3-(azepan-1-ylmethyl)-1~{H}-indole 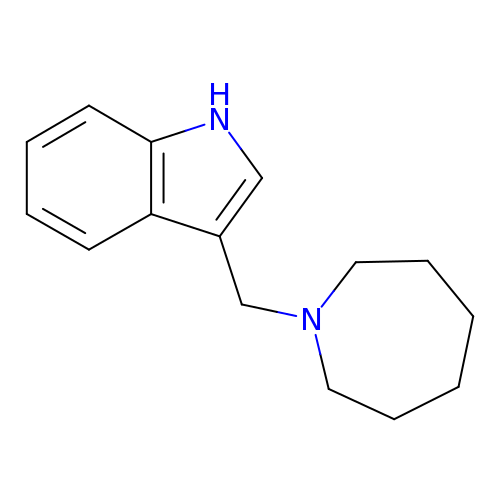| C15 H20 N2 | PDUPXVBNXBQTQH-UHFFFAOYSA-N>MKHLEEKTLSTRQIFKGRYLKIEQDQVQAPDGRTYTREYILHPGAAMMIPLLPNGNVVMIHQYRHAVKKVFLEFPAGKRDHNEETLLTAKRELLEETGYEAKDWKFLTTIHPVIGYSNEHIDLYLARDLTHLEQRLDQGEFIEVVEVKPADLMQLVLEGKVSDVKT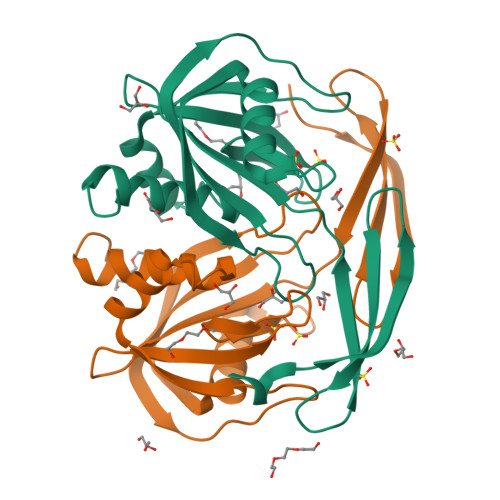QIGAFWLDKFLRGEWN[2x]>[2x]MKKRAIQKIISSIVSLAVLTSVPVMQKPSVLAASSDSTSASKTDFFSSFEKSDLQLTWTNTVETDANGKKMSSGIDGNVKRDLILGDITDKVVQVTASANNPPNEIDSKLIDGDPTTKWLAFEPTANIVLKLAEPVAVVKYALTSANDAKGRDPKNWTLYGSLDGTNWTAVDTREGEDFKDRFQRNMYDLKNTTKYLYYKLDITKNAGDSITQLAEISLSDGIEVPAPPPGDMKSLIGKGPTSSYTAKTNVGWTGLGALNYSGTHLSDGRAYSYNKLYDVDILVTPATELSYFIAPEFTDKNHNDYSSTYVSVDLAFSDGTYLHDLKAVDQYGVGLNPKDQGDSKYLYVNQWNTIKSTIGSVAAGKTIKRILVAYDNPKGPGAFRGSIDDIKIDGKPVQKAFGSPIDYVNILRGTQSNGSFSRGNNFPAVAIPHGFNFWTPTTNAGSSWIYQYHESNSVNNLPQIQAFSVSHEPSPWMGDRQTFQVMPSASTAATPNANRDSRALEFNHANEIAQPHYYSVKFENGIRTEMTPTDHAAMFKFTFTGATSNLIFDNVNNNGGLTIDAKSGEITGYSDVKSGLSTGATRLFVYAAFDKPVIKSGKLTGESRNNVTGYVRFDTSKDEDKVVTMKIATSLISVEQAKKNLEQEIGLNDTFEGLKEKAKTEWNKKLGIIEVEGASEDQLVTLYSNLYRLFLYPNSAFENVGTTTDPVYKYASPYSAATGQDTATTTGAKIVDGKTYVNNGFWDTYRTAWPAYSLLTPTFAGELIDGFVQQYRDGGWIARWSSPGFANLMPGTSSDVAFADAYLKGVTNFDVQSFYQSAIRNAEAVSPNAGTGRKGLTTSIFDGYTNTSTGEGLAWAMDGYINDFGIANLAKALKEKGDKSDPYYANYAADYQYFLNRAQNYVHMFNPSIEFFNGRTANGAWRSTPDNFNPAVWGSDYTETNGWNMAFHVPQDGQGLANLYGGKEGLATKLDQFFSTSETGLFPGSYGGTIHEMREARDVRMGMYGHSNQPSHHIAYMYDYAGQPWKTQEKVREALNRLYIGSAIGQGYSGDEDNGEMSAWYILSAMGFYPLKMGTPEYAIGAPLFKKATIHLENGKSIVINAPNNSKENKYVQSMKVNGKAYAKTSILHADIANGAVIDFEMGSKPSKWGSGDQDILQSITPGSTDGTSLSPLPLRDVTDRLIAAEKGAVTVSDEGNGQLLFDNTSNTQLSMKSKTPSIVYQFKEGKQNVKMYTLTSSKASQNEDPKSWVLKGSNDGKSWSVLDQRKNETFQWRQYTRAFTIQHPGKYSQYKLEITENAGAEVTTLAELELLGYDDVTNSYQAVYELMEQFKQSKDLTGPMAVQLNNSLTTSLDHFKKDHKDQAIKHLEDFLKHLNNKGLQDRISSKAKGVLSADANQLIVLLARD

Here, we report the biochemical characterization and the crystal structure of the full-length multi-domain GH92 α-mannosidase from Neobacillus novalis (NnGH92), a bacterium identified in agricultural soils. All known family GH92 members are Ca2+-dependent exo-α-mannosidases that perform the hydrolysis of terminal non­reducing mannose residues with inversion of the anomeric configuration. All known structures of GH92 α-mannosidase catalytic domains have a highly conserved two-subdomain composition, a N-terminal β-sandwich and a C-terminal (α/α)6-barrel, with both subdomains contributing to a pocket-like active site with distinctive −1 and +1 sugar-binding subsites. In contrast to B. thetaiota­omicron, which produces GH92 α-mannosidases as solely catalytic domains, NnGH92 has five domains.

Here, the biochemical investigation and crystal structure of the full-length five-domain GH92 α-1,2-mannosidase from Neobacillus novalis (NnGH92) with manno­imidazole bound in the active site and an additional mannoimidazole bound to the N-terminal CBM32 are reported. NnGH92 only crystallized in the presence of ManI, suggesting that the ligand binding improved the structure stability, leading to the formation of high-quality crystals. There are two independent monomers in the asymmetric unit. In chain B, there were only very poor fragments of density for the N-terminal CBM32 domain, and residues 79–227 are missing from the model. At the N-terminus there is the start of an all-β-sheet domain reminiscent of a CBM and termed ‘CBM-like’, which is made up of residues 42–77 and 259–395. A CBM32 (residues 86–222) is inserted into a loop of the CBM-like domain. These are followed by the catalytic domain (residues 408–1166), the C-terminal CBM32 (residues 1182–1316) and a four-helix bundle domain (FHB; residues 1321–1411). The rest of the description will focus on the better ordered chain A. The catalytic domain was traced without any breaks and its fold, as expected, was very similar to that of Bt3990, with an r.m.s.d. of 2.01 Å over 712 equivalent Cα atoms reflecting the moderate sequence identity (41.6%). The reaction mechanism of GH92 enzymes, with catalysis occurring with inversion of the anomeric configuration, requires two residues: an acid to assist the departure of the leaving group and a base to enhance the nucleophilic attack of water. The catalytic residues, the Brønsted acid Glu944 (Glu533 in Bt3990) and the Brønsted base Asp1058 (Asp644 in Bt3990), are conserved. The specificity of the α-1,2-mannosidase Bt3990 is primarily driven by three residues at the +1 subsite: the His584-Glu585 pair of residues forming hydrogen bonds to O3 and O4 of the MSM mannose and Trp88 providing a hydrophobic interaction.>EKAVLEQFGFPLTGTEARCYTNHALSYDQAKRVPRWVLEHISKSKIMGDADRKHCKFKPDPNIPPTFSAFNEDYVGSGWSRGHMAPAGNNKFSSKAMAETFYLSNIVPQDFDNNSGYWNRIEMYCRELTERFEDVWVVSGPLTLPQTRGDGKKIVSYQVIGEDNVAVPSHLYKVILARRSSVSTEPLALGAFVVPNEAIGFQPQLTEFQVSLQDLEKLSGLVFFPHLDRTSDIRNICSVDTC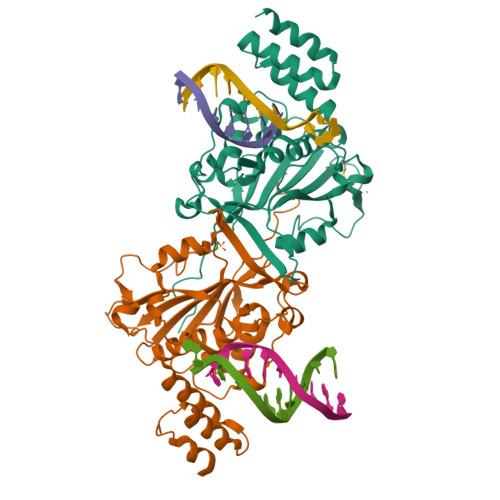KLLDFQEFTLYLSTRKIEGARSVLRLEKIMENLKNAEIEPDDYFMSRYEKKLEELKAKEQSGTQIRKPS[4x]>AQYEDGKQYTTLEKPVAGAPQVLEFFSFFCGHAYQFEEVLHISDNV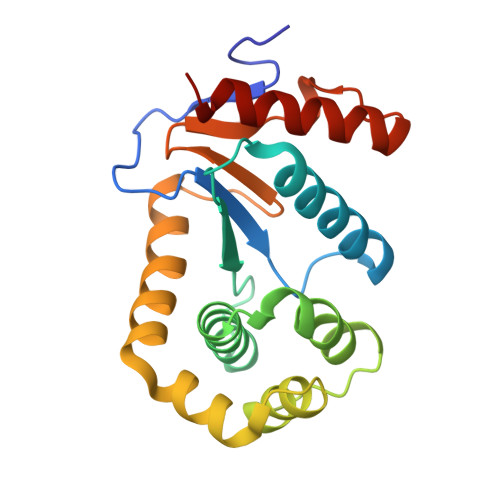KKKLPEGVKMTKYHVNFMGGDLGKDLTQAWAVAMALGVEDKVTVPLFEGVQKTQTIRSASDIRDVFINAGIKGEEYDAAWNSFVVKSLVAQQEKAAADVQLRGVPAMFVNGKYQLNPQGMDTSNMDVFVQQYADTVKYLSEKK[2x]>QPSFRPSALVVPVKKDASTLQYVTTINQRTPLVSENLVVDLGGRFLWVDCDQNYVSSTYRPVRCRTSQCSLSGSIACGDCFNGPRPGCNNNTCGVFPENPVINTATGGEVAEDVVSVESTDGSSSGRVVTVPRFIFSCAPTSLLQNLASGVVGMAGLGRTRIALPSQFASA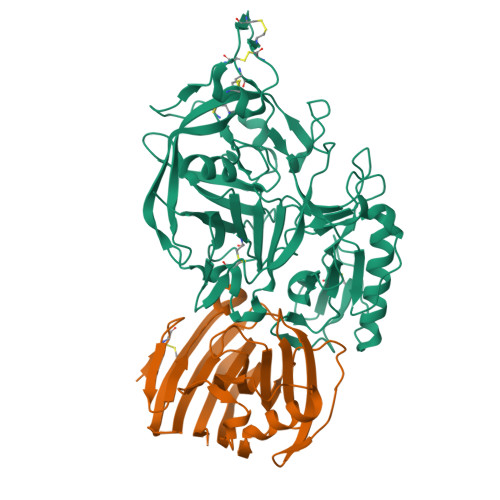FSFKRKFAMCLSGSTSSNSVIIFGNDPYTFLPNIIVSDKTLTYTPLLTNPVSTSATSTQGEPSVEYFIGVKSIKINSKIVALNTSLLSISSAGLGGTKISTINPYTVLETSIYKAVTEAFIKESAARNITRVASVAPFGACFSTDNILSTRLGPSVPSIDLVLQSESVVWTITGSNSMVYINDNVVCLGVVDGGSNLRTSIVIGGHQLEDNLVQFDLATSRVGFSGTLLGSRTTCANFNFTS[2x];>GPLGSDFCGQWDTATAGDFTLYNDLWGESAGTGSQCTGVDSYSGDTIAWHTSWSWSGGSSSVKSYVNAALTFTPTQLNCISSIPTTWKWSYSGSSIVADVAYDTFLAETASGSSKYEIMVWLAALGGAGPISSTGSTIATPTIAGVNWKLYSGPNGDTTVYSFVADSTTESFSGDLNDFFTYLVDNEGVSDELYLTTLEAGTEPFTGSNAKLTVSEYSISIE[2x]> SMTRPRLYEEAVKRLHAEARKAGVNLDKTFNASEMSYIIEEVYV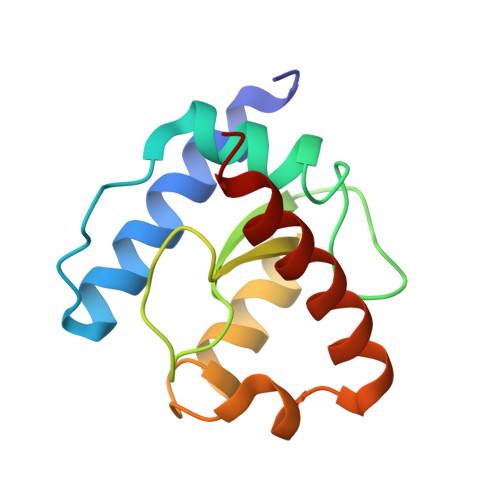GRSALPPHESQKVTVVRWNPQLPFDHTNLVAMTRNEARYHEDNVLAKNVDPSTVYGKDVIEVVHSFLRRLRMWEMLY> TPVSEKQLAEVVANTVTPLMKAQSVPGMAVAVIYQGKPHYYTFGKADIAANKPVTPQTLFELGSISKTFTGVLGGDAIARGEISLDDPVTRYWPQLTGKQWQGIRMLDLATYTAGGLPLQVPDEVTDNASLLRFYQNWQPQWKPGTTRLYAGASIGLFGALAVKPSGMPYEQAMTTRVLKPLKLDHTWINVPKAEEAHYAWGYRDGKAVRVSPGMLDAQAYGVKTNVQDMANW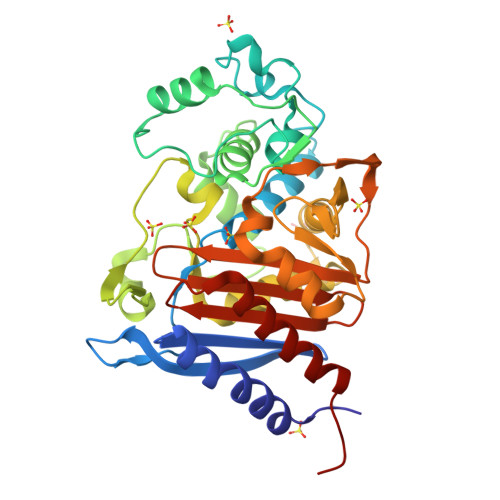VMANMAPENVADASLKQGIALAQSRYWRIGSMYQGLGWEMLNWPVEANTVVEGSDSKVALAPLPVVEVNPPAPPVKASWVHKTGSTGGFGSYVAFIPEKQIGIVMLANTSYPNPARVEAAYHILEALQHHHHHH>[4x]AAPPRGRILGGREAEAHARPYMASVQLNGAH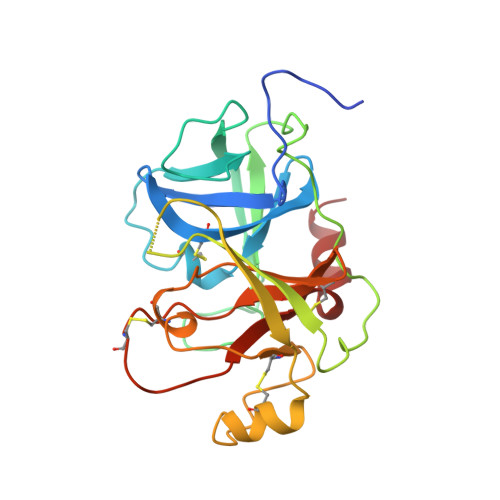LCGGVLVAEQWVLSAAHCLEDAADGKVQVLLGAHSLSQPEPSKRLYDVLRAVPHPDSQPDTIDHDLLLLQLSEKATLGPAVRPLPWQRVDRDVAPGTLCDVAGWGIVNHAGRRPDSLQHVLLPVLDRATCNRRTHHDGAITERLMCAESNRRDSCKGDSGGPLVCGGVLEGVVTSGSRVCGNRKKPGIYTRVASYAAWIDSVLA>[2x]MGSKFIQNAAEIAKK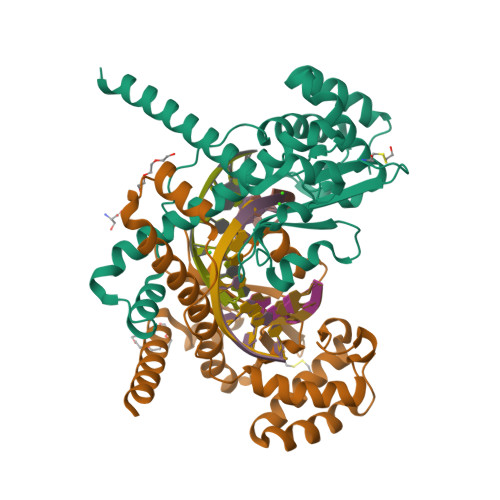AMDSVDPSLSEKFTIVIRFLTDNPDAASALKGKERSIVGTEEYIIASATNFKKGRDPRTPLPPSTIPDEMVSVILNKYFEVPSEELEKAEEWHRLSMGAENIVGDLLERYIAEVIEPHGWIWCSGSMVRAVDFIYCDSENVWQSLQVKNRDNTENSSSAAIRHGTPIKKWFRTFSKKRGDNWDKFPSLEGKENLSEKGFKLYVEKYLSALRAIKALEHHHHHH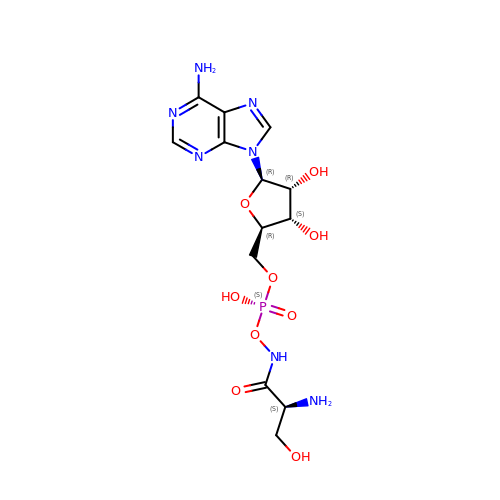SERYL-HYDROXAMATE-ADENOSINE MONOPHOSPHATE | C13 H20 N7 O9 P | WBBUFKBXWUDMQG-YTMOPEAISA-N> MKLDIKKTFSNRSDRVKGIDFHPTEPWVLTTLYSGRV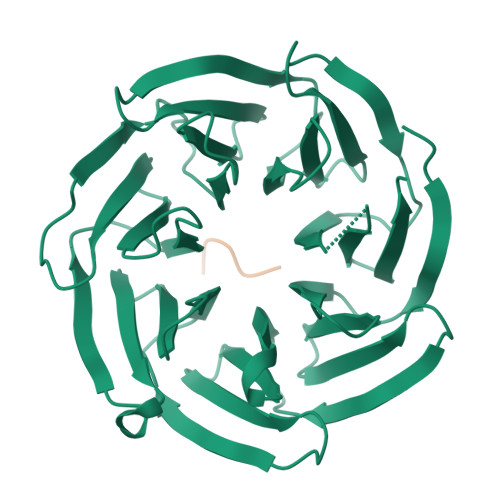EIWNYETQVEVRSIQVTETPVRAGKFIARKNWIIVGSDDFRIRVFNYNTGEKVVDFEAHPDYIRSIAVHPTKPYVLSGSDDLTVKLWNWENNWALEQTFEGHEHFVMCVAFNPKDPSTFASGCLDRTVKVWSLGQSTPNFTLTTGQERGVNYVDYYPLPDKPYMITASDDLTIKIWDYQTKSCVATLEGHMSNVSFAVFHPTLPIIISGSEDGTLKIWNSSTYKVEKTLNVGLERSWCIATHPTGRKNYIASGFDNGFTVLSLG;> AKEKSD>[2x]STRDYEIQRERIELGRCIGEGQFGDVHQGIYMSPENPAMAVAIKTCKNCTSDSVREKFLQEALTMRQFDHPHIVKLIGVITENPVWIIMELCTLGELRSFLQVRKFSLDLASLILYAYQLSTALAYLESKRFVHRDIAARNVLVSATDCVKLGDF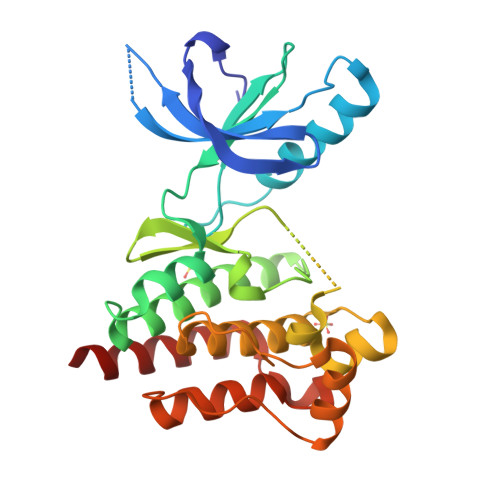GLSRYMEDSTYYKASKGKLPIKWMAPESINFRRFTSASDVWMFGVCMWEILMHGVKPFQGVKNNDVIGRIENGERLPMPPNCPPTLYSLMTKCWAYDPSRRPRFTELKAQLSTILEEEKLQ> MGVEKVPKYDIPVKKVEYVFIELDKMKPHEQLVQRELEDFIESVTGSGIFWKPMLLAKIPGTDEYLIVDGHHRWAGLQKLGAKRAPSVILDYFDEGVKVYTWYPAFKGDVNKVIERLKAEGLEVIEDEKAEEKAEKGEIAFALIGEKSFAIPGGLEEQKKVSKVLDEMDQAKEIELVYYGLKEDAKADMEKGEIDYVFIRKAPTKEEVMELVKRGEVFSPKTTRHVLPFIPDKIDVKLEDLF

A 26 kD nuclease from Pyrococcus furiosus used in the current study had resisted crystallization inspite of extensive purification and crystallization space screening. Here, we report the successful crystallization of a nuclease employing a reductive methylation protocol. The key to crystallization was the successful introduction of 44 new cohesive (NZ) CH...O contacts (3.2 – 3.7 Å) by the addition of 2 methyl groups to the side chain amine nitrogen (NZ) of 9 lysine residues of the nuclease. The new contacts dramatically altered the crystallization properties of the protein, resulting in crystals that diffracted to 1.2 Å resolution.

After purifying the protein to homogeneity, two methyl groups were covalently linked to the free amine nitrogen of lysine residues by treating the protein with formaldehyde and dimethylamine borane complex (DMAB). Electron density for only 9 amine nitrogens out of 32 (including the N-terminal amine group), could be unambiguously assigned as dimethylated. Forty new intra molecular (NZ)CH...O contacts in the range 3.2 to 4.0 Å were generated because of the methylation, of which 25 interactions were between 3.2 to 3.8 Å. The methyl carbons of all the dimethylated lysine residues were involved in the formation of multiple new symmetry-generated intermolecular contacts. The structure reveals 96 new symmetry-generated inter molecular contacts in the range 3.2 – 5.0 Å involving the (NZ)CH group and 28 of these inter molecular contacts are of the (NZ)CH...O type and in the range 3.2 – 4.0 Å. Analytical ultracentrifugation analysis and thermodynamics results revealed a more compact protein structure with better solvent exclusion of buried Trp residues in the folded state of the methylated protein, assisting crystallization. Interestingly, we found that the chemical modification resulted in a decrease in the mid-point of unfolding in both GdmCl and thermal denaturation, which corresponds to a decrease in the free energy of unfolding, Δ GU,H20, of 18 ± 3 kJ/mol. The only short contacts – a 3.0 Å link between the CH2 methyl carbon of MLY221 and a phosphate oxygen, and a 3.1 Å bond between the carboxyl oxygens of E36 and the MLY221 methyl carbons, resulted in the distortion of the conformation of the MLY221 and the glutamic acid, suggesting steric clashes due to the excessive closeness of the methyl carbon and the oxygen atoms. The methylated protein lost its ability to cleave DNA (results not shown). The dimethylation of K221 sitting at the edge of the active site may sterically hinder access of the active site to the incoming DNA.> SYHLDTTAPPPTNLSTLPNNTLFHLWRPRAHILPAEGQIGDPCAHYTDPSTGLFHVGFLHDGDGIAGATTANLATYTDTSDNGSFLIQPGGKNDPVAVFDGAVIPVGVNNTPTLLYTSVSFLPIHWSIPYTRGSETQSLAVARDGGRRFDKLDQGPVIADHPFAVDVTAFRAPFVFRSARLDVLLSLDEEVARNETAVQQAVDGWTEKNAPWYVAVSGGVHGVGPAQFLYRQNGGNASEFQYWEYLGEWWQEATNSSWGDEGTWAGRWGFNFETGNVLFLTEEGHDPQTGEVFVTLGTEGSGLPIVPQVSSIHDMLWAAGEVGVGSEQEGAKVEFSPSMAGFLDWGFSAYAAAGKVLPASSAVSKTSGVEVDRYVSFVWLTGDQYEQADGFPTAQQGWTGSLLLPRELKVQTVENVVDNELVREEGVSWVVGESDNQTATLRTLGITIARETKAALLANGSVTAEEDRTLQTAAVVPFAQSPSSKFFVLTAQ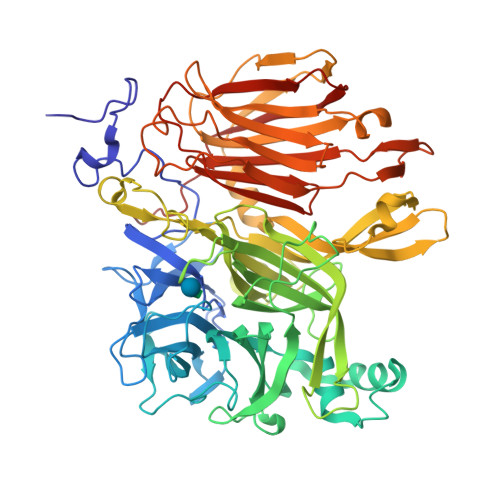LEFPASARSSPLQSGFEILASELERTAIYYQFSNESLVVDRSQTSAAAPTNPGLDSFTESGKLRLFDVIENGQEQVETLDLTVVVDNAVVEVYANGRFALSTWARSWYDNSTQIRFFHNGEGEVQFRNVSVSEGLYNAWPER> GSSGSSGLSDFSWSQ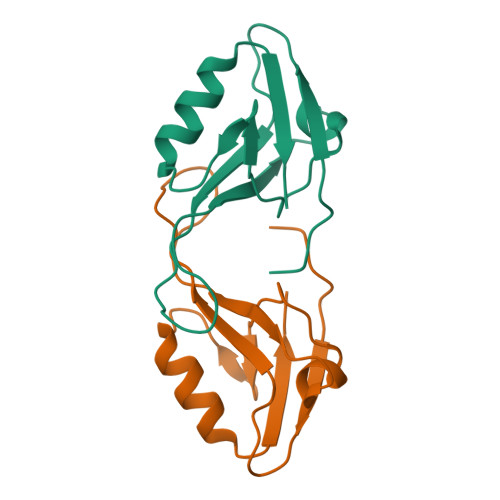RKLVTVEKQDNETFGFEIQSYRPQNQNACSSEMFTLICKIQEDSPAHCAGLQAGDVLANINGVSTEGFTYKQVVDLIRSSGNLLTIETL> MMQQSRPASDPQVVEAARKEGRLIIYSSTDQSSAQALLDDFRKLYPFIQIEYNDLGTQAIYDRFVSETAAGASSADLLWSSAMELQVKLASEGYALPYDSPEAKNWPANARLGNLAYSTTLEPAVVVYNKRFLKPEEVPTTREG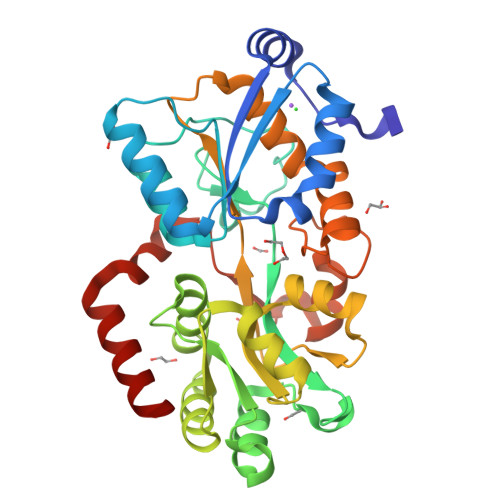LARLLQEPRMRGRVATWDPERSAVGFTILKADYDRFPAFQELARAFGKAQAALYSSAGAAFEKVISGEHYLAYGFFGSYALLRQRTVKDLGIAYLTDGTVAIQRVAFINKRAAHPNAAKLFLDYLLSLRGQNLMAYTALIFARRETVVGEATPQALYKAVGGKDKVYAIPVSTEILKNLDPAERMRFLTFWRQAVRGQ>[2x]FQHMGTVSWNLREMLAHAEETRKLMPVCVETK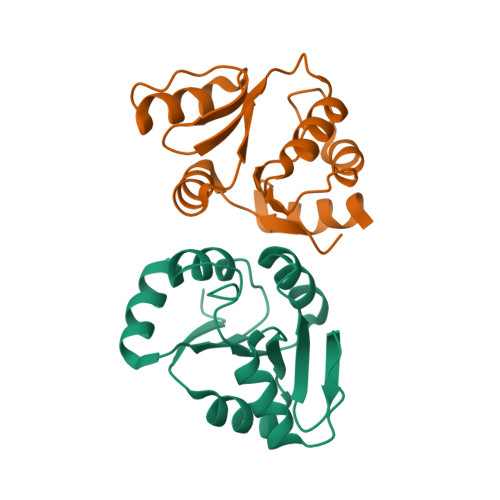AIVSTIQRKYKGIKIQEGVVDYGARFYFYTSKTTVASLINTLNDLNETLVTMPLGYVTHGLNLEEAARYMRSLKVPATVSVSSPDAVTAYNGYLT>[2x]MATERQAAIAKKRQTDKALNKKAALKNSQLSRKINQTTFSNNKNTDEQVTKALNLSHFVGSALVVKNDHVIYNRAFGYANKAKNQRNKVNSKYQILSIQKSMTAVGIMQLVQAGKVKLTDPISKYYPTLKHGRQTTLRQMLDMTTGFRLKSGSKEFLPENQVIDFAAHNVFYYPDKNGIYNYSSVNFLLLAGIIRKVTGQSYQHFFTTHFIDKLNLNETGFLIHGQGQDATTGYRALADQTLPNYDQTMPESKSQMANELGTGQVYMSTADLFTVESAILKGQLLSKKNVAILHTRTATGEYGGGVYNMSNGIRSHGLGYGYESSIFLSPDGKTGVVLMSNYYRKAAGIQATANKIFTELMKGDIKLEHHHHHH

We show that lipoteichoic acids (LTAs) but not wall teichoic acids are D-alanylated in Lactiplantibacillus plantarumNC8 cell envelope and demonstrate that DltE is a D-Ala carboxyesterase removing D-Ala from LTA. (a) The dltE gene encodes for a 397 residues protein composed of a transmembrane segment predicted between residues 12 and 34 and a larger C-terminal extracellular region from residues 34–397 and named DltEextra. The domain consists of two subdomains, an α-β sandwich (residues 76–126 and 246–397) that form a five strand (β1–β5) antiparallel β-sheet flanked by 5 α-helices (α2, α9–α12) and an α-helix-rich region (residues 127–245) folding in 6 α-helices (α3-α8). DltE is structurally homologous to the D-Ala-D-Ala carboxypeptidase R61 (DDCP) from Streptomyces (Kelly et al., 1986; McDonough et al., 2002) that exhibits the classical β-lactamase fold of PBPs.

The first motif is strictly conserved in DltE (128SIQK131) and located as for DDCP at the beginning of the α-helix-rich region (α3 helix in DltE, α2 in DDCP) at the interface with the β-sheet. The positions of the active site S-X-X-K motif (128SIQK131), containing the catalytic Ser128 and Lys131 residues, and the catalytic Tyr213 from the second motif are conserved. The position of the catalytic Tyr213 from the second motif is also conserved and found in the loop connecting α5 and α6, close to the catalytic dyad. In contrast, several striking features distinguish DltE from DDCP and more generally from PBPs and DD-carboxypeptidases. The β3-strand that usually bears the third motif and defines one side of the catalytic cavity is not conserved in terms of length and position (McDonough et al., 2002). The global architecture of the active site cavity of DltE is therefore reshaped and different from that of DDCP enzymes, adopting a deeper cleft topology largely opened on both sides of the protein. The catalytic Ser, colored in red, is buried at the bottom of the catalytic cavity in DDCP and lying in the middle of a large cleft in DltE.>TYLDRLALRYDREGEPSQLAAVDIFVSTVDPLKEPPLVTANTVLSILAVDYPVDKVSCYVSDDGAAMLSFESLAETSEFARKWVPFCKKYSIEPRAPEWYFAAKIDYLKDKVQTSFVKDRRAMKREYEEFKIRINALVSKALKCPEEGWVMQDGTPWPGNNTRDHPGMIQVFLGQNGGLDAEGNELPRLVYVSREKRPGFQHHKKAGAMNALVRVSAVLTNGPFILNLDCDHYINNSKALREAMCFLMDPNLGKQVCYVQFPQRFDGIDKNDRYANRNTVFFDINLRGLDGIQGPVYVGTGCVFNRTALYGYEPGSGSGSLEKRFGQSAVFVASTLM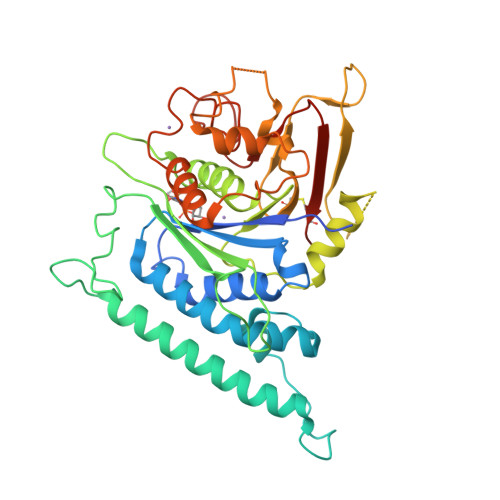ENGGVPPSATPENLLKEAIHVISCGYEDKSDWGMEIGWIYGSVTEDILTGFKMHARGWRSIYCMPKLPAFKGS[2x]> MGSDAFDEMDEIWALYADDGAQALDAMEASLLALQAGEDAAAHVGPLFRAVHTFKGNS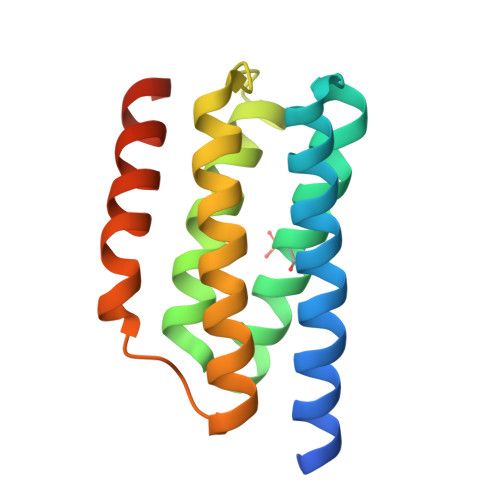RVLGLSVVESRAHLCEDLIGLVRDAGVPMDGEIVEILLFASDTLRAMLEETAASRADVEGTGSEALMDQLRSKIARCSRSHHHHHH>GSSHHHHHHSSGLVPGGSHMVSKGEENNMAVIKPDMKIKLRMEGAVNGHPFAIEGVGLGKPFEGKQSMDLKVKEGGPLPFAYDILTTVFXNRVFAKYPENIVDYFKQSFPEGYSWERSMNYEDGGICNATNDITLDGDCYIYEIRFDGVNFPANGPVMQKRTVKWEPSTEKLYVRDGVLKGDVNTALSLEGGGHYRCDFKTTYKAKKVVQLPDYHFVDHHIEIKSHDK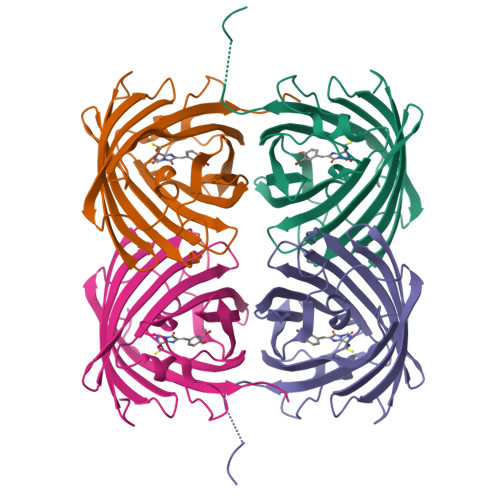DYSNVNLHEHAEAHSGLPRQAMDELYK[8x]> GSLIGLMKDAFQPHHHHHHHLSPHPPGTVDKKMVEKCWKLMDKVVRLCQNPKLALKNSPPYILDLLPDTYQHLRTILSRYEGKMETLGENEYFRVFMENLMKKTKQTISLFKEGKERMYEENSQPRRNLTKLSLIFSHMLAELKGIFPSGLFQGDTFRITKADAAEFWRKAFGEKTIVPWKSFRQALHEVHPISSGLEAMALKSTIDLTCNDYISVFEFDIFTRLFQPWSSLLRNWNSLAVTHPGYMAFLTYDEVKARLQKFIHKPGSYIFRLSCTRLGQWAIGYVTADGNILQTIPHNKPLFQALIDGFREGFYLFPDGRNQNPD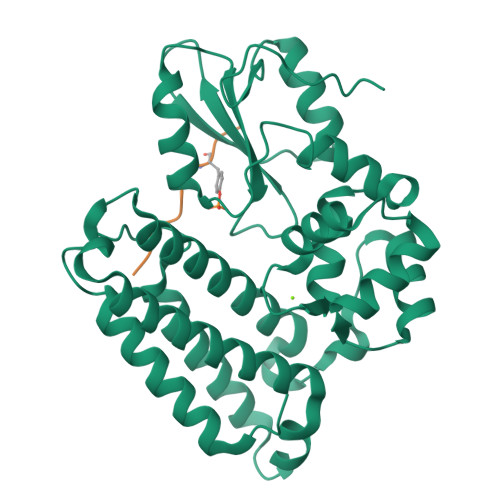LTG;> GRARAVENQYSFY>MGHHHHHHTQILIVEDEQNLARFLELELTHENYNVDTEYDGQDGLDKALSHYYDLIILDLMLPSINGLEICRKIRQQQSTPIIIITAKS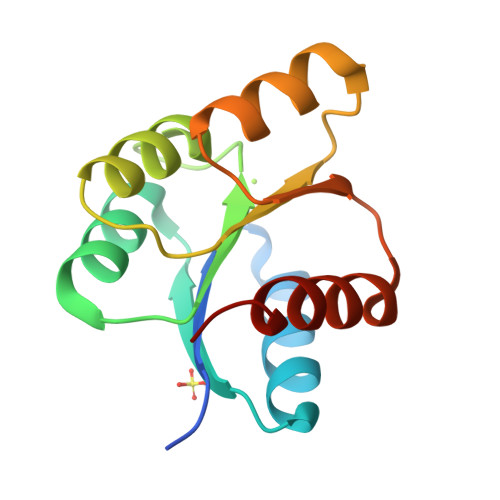DTYDKVAGLDYGADDYIVKPFDIEELLARIRAILRRQPQ[4x]>[3x]MHHHHHHSLLTEVETYVLSIVPSGPLKAEIAQRLEDVFAGKNTDLEVLMEWLKTRPILSPLTKGILGFVFTLTVPSERGLQRRRFVQNALNGNEDPNNMDKAVKLYSK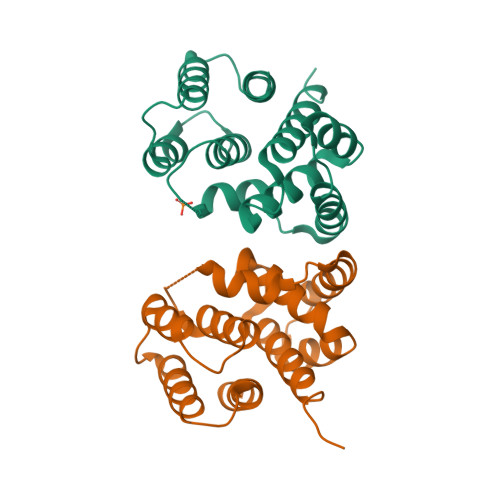LKSEITFHGAKEIALSYSAGALASCMGLIYNRMGAVTTEVAFGLVCATCEQIADSQHRSHRQM> ASAKELACQEITVPLCKGIGYQYTYMPNQFNHDTQDEAGLEVHQFWPLVEIQCSPDLKFFLCSMYTPICLEDYKKPLPPCRS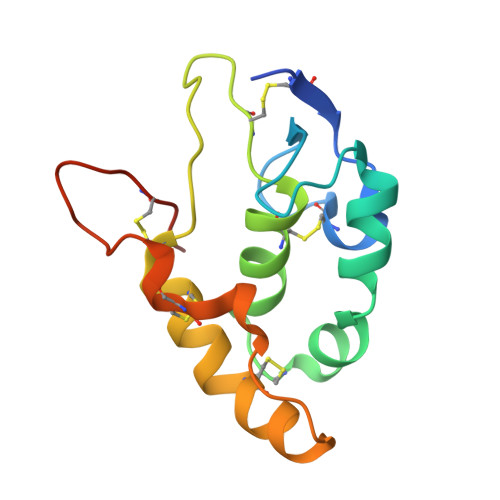VCERAKAGCAPLMRQYGFAWPDRMRCDRLPEQGNPDTLCMDHHHHHH> V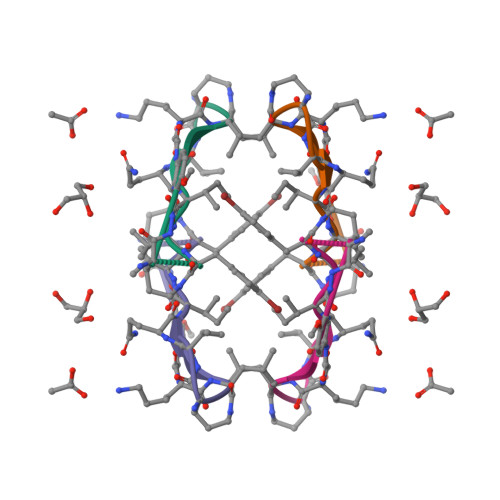QIVYAXKLA5-[1-(pyridin-2-ylmethyl)indol-6-yl]-1~{H}-pyrazol-3-amine 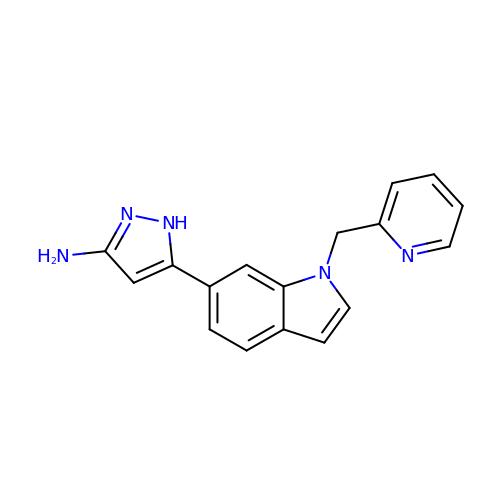| C17 H15 N5 | QCOOOKJAGFXTOZ-UHFFFAOYSA-N>MKGTIVGTWIKTLRDLYGNDVVDESLKSVGWEPDRVITPLEDIDDDEVRRIFAKVSEKTGKNVNEIWREVGRQNIKTFSEWFPSYFAGRRLVNFLMMMDEVGLQLTKMIKGATPPRLIAKPVAKDAIEMEYVSKRKMYDYFLGLIEGSSKFFKEEISVEEVERGEKDGFSRLKVRIKFKNPVFEYK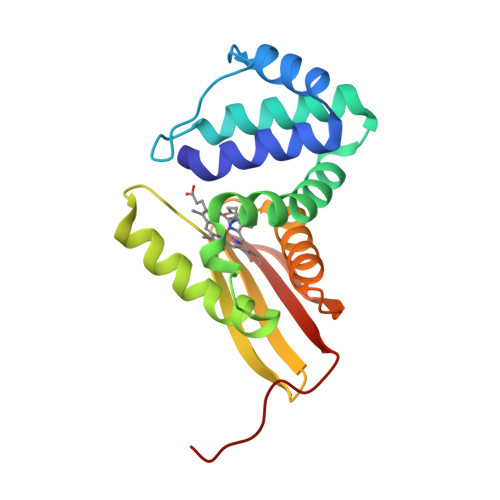KN[2x]> MAQQANVGELLAMLDSPMLGVRDDVTAVFKENLNSDRGPMLVNTLVDYYLETSSQPALHILTTLQEPHDKHLLDRINEYVGKAATRLSILSLLGHVIRLQPSWKHKLSQAPLLPSLLKCLKMDTDVVVLTTGVLVLITMLPMIPQSGKQHLLDFFDIFGRLSSWCLKKPGHVAEVYLVHLHASVYALFHRLYGMYPCNFVSFLRSHYSMKENLETFEEVVKPMMEHVRIHPELVTGSKDHELDPRRWKRLETHDVVIECAKISLDPTEASYEDGYSVSHQISARFPHRSADVTTSPYADTQNSYGCATSTPYSTSRLMLLNMPGQLPQTLSSPSTRLITEPPQATLWSPSMVCGMTTPPTSPGNVPPDLSHPYSKVFGTTAGGKGTPLGTPATSPPPAPLCHSDDYVHISLPQATVTPPRKEERMDSARPCLHRQHHLLNDRGSEEPPGSKGSVTLSDLPGFLGDLASEEDSIEKDKEEAAISRELSEITTAEAEPVVPRGGFDSPFYRDSLPGSQRKTHSAASSSQGASVNPEPLHSSLDKLGPDTPKQAFTPIDLPCGSADESPAGDRECQTSLETSIFTPSPCKIPPPTRVGFGSGQPPPYDHLFEVALPKTAHHFVIRKTEELLKKAKGNTEEDGVPSTSPMEVLDRLIQQGADAHSKELNKLPLPSKSVDWTHFGGSPPSDEIRTLRDQLLLLHNQLLYERFKRQQHALRNRRLLRKVIKAAALEEHNAAMKDQLKLQEKDIQMWKVSLQKEQARYNQLQEQRDTMVTKLHSQIRQLQHDREEFYNQSQELQTKLEDCRNMIAELRIELKKANNKVCHTELLLSQVSQKLSNSESVQQQMEFLNRQLLVLGEVNELYLEQLQNKHSDTTKEVEMMKAAYRKELEKNRSHVLQQTQRLDTSQKRILELESHLAKKDHLLLEQKKYLEDVKLQARGQLQAAESRYEAQKRITQVFELEILDLYGRLEKDGLLKKLEEEKAEAAEAAEERLDCCNDGCSDSMVGHNEEASGHNGETKTPRPSSARGSSGSRGGGGSSSSSSELSTPEKPPHQRAGPFSSRWETT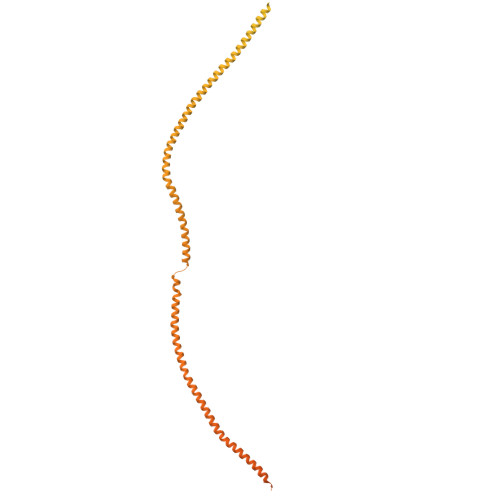MGEASASIPTTVGSLPSSKSFLGMKARELFRNKSESQCDEDGMTSSLSESLKTELGKDLGVEAKIPLNLDGPHPSPPTPDSVGQLHIMDYNETHHEHS> PAAAPGKNFDLSHWKLQLPDANTTEISSANLGLGYTSQYFYTDTDGAMTFWAPTTGGTTANSSYPRSELREMLDPSNSKVNWGWQGTHTMKLSGKTVQLPSSGKIIVAQIHGIMDDGTNAPPLVKAVFQDGQLDMQVKQNSDGTGSDVHNYFTGIKLGDLYNMEIRVTDGVAYVTMNGDTRSVDFVGKDAGWKNLKYYFKAGNFVQDNTSTGGSA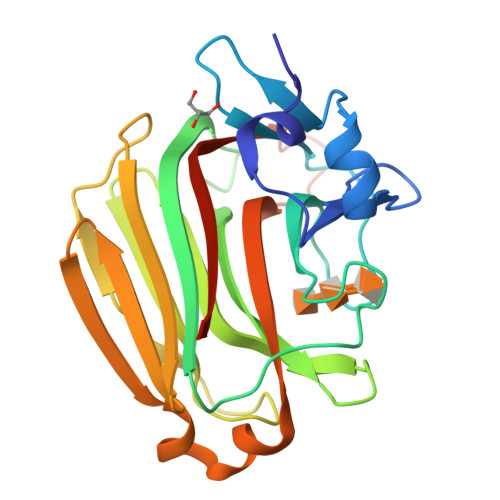IAKLYSLSVSHSNLEHHHHHH> MRGSHHHHHHGSMDYKRRIHKFQAHFGKKGFEGALVAPGSNFYYLTGFNPLGTLE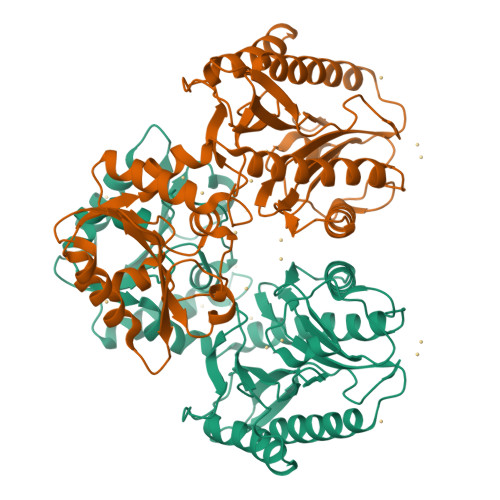RLFVLILPSEGLLTAIAPRLYEKELEEFNGEVVLWSDSENPYKIFATKIKETFKEGEKLLIDDTMPVGVFLKAKDIFDKYSLHPISPVISELREIKDKDEIKAHKKAAEIVDKVFYRFIEGKLEGKSERELANRIEYMIKNEFGADDVSFEPIVASGPNGANPHHRPSHRKIRKGDVVIFDYGAKYLGYCSDVTRTVVVGPPSEEVKKVYEIVKEAQETAVQKVAEGIPAEVVDATARGIISKYGYGEYFIHRTGHGLGIDVHEEPYISPGNKKILKDGMVFTIEPGIYLQGKFGVRIEDDVALVDKKGIRLTNADRELITL> MSGEEERKEKREKVRAGLKRAIAELPAEVAARCLALLDDASDEEFIEAVLEVLEAMREALVAMAR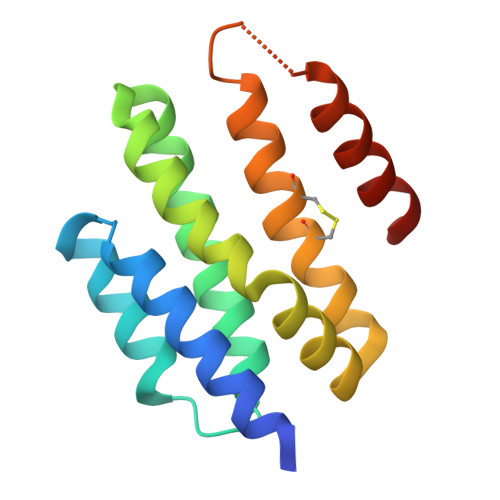EGRLDAVRRATSHINEVLVDAAELALEKGREYFRRLCLIVCDMMIELIRLEPEQTPELRRIRERLEEIRRRLEGSG(Z)-2-[4-(1,2)-DIPHENYL-1-BUTENYL)-PHENOXY]-N,N-DIMETHYLETHANAMINE 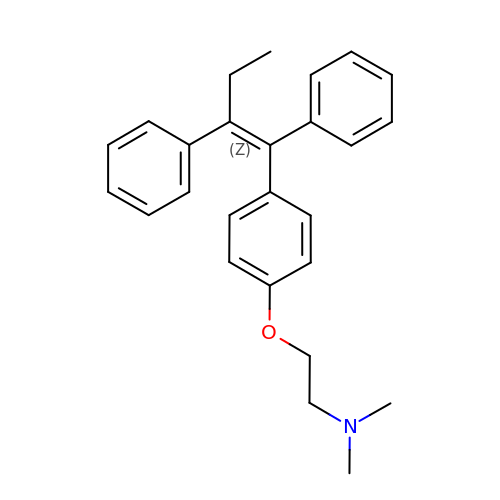| C26 H29 N O | NKANXQFJJICGDU-QPLCGJKRSA-N>[2x]MGYIIDQDTPEYVSVKYKSVYAIEDSWVRDGDYANTNYGTANTLVVKKDGDGYNREAYIKFDLQNIDITKYQNIFLALYVANSNTSIHDTQWNIGYVADNTWSEKSITW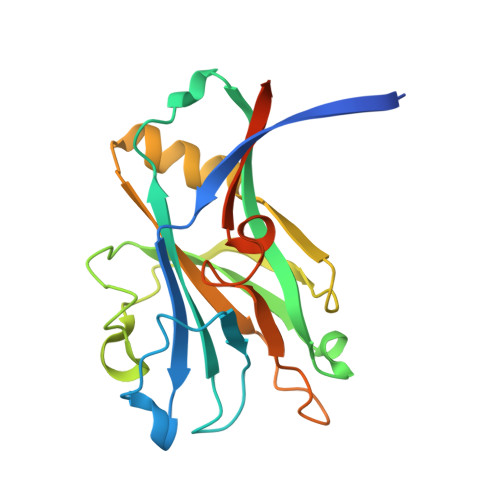NNRPVTTNTIATVSTVPAGSNVMVDISQAVFNEIKNNSKTLTLHISSTTRGADGKTDAQFYSKEGSDPLKAPQLMLQEKGESNTASLEHHHHHH8-(3-{[(2S)-1-aminopropan-2-yl]oxy}benzyl)-4-(cyclohexylamino)-1-(3-fluorophenyl)-1,3,8-triazaspiro[4.5]dec-3-en-2-one 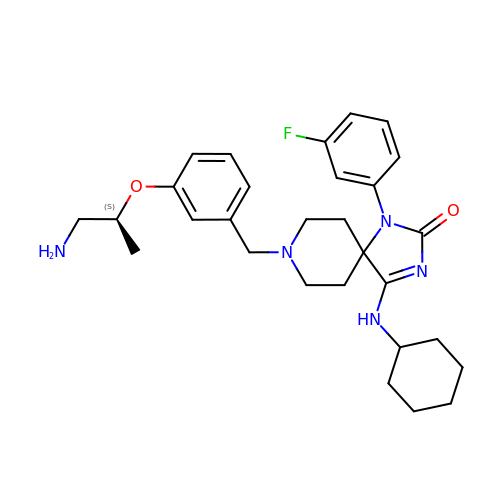| C29 H38 F N5 O2 | GJCCGBZILLQLCV-NRFANRHFSA-N>[4x]MTDYDLAKETAAWLNKQLQIRPVLGIVCGSGLGKIGDSLETSITVAYSDIPNFPVGSVKGHAGSLIFGSVNGVSCVCMKGRFHLYEGHTAARATFPMRVFKALGVKIV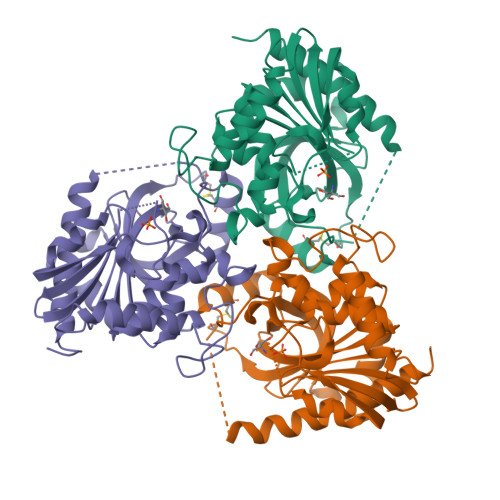VLTNAAGGLNPSYRPGDFMVVRDHINLPGLAGANPLTGPNDDTEGERFPSMTSVYDKTLRKYAISAARELGMSYATHEGVYCCVNGPSFETPAECKILRLMGSDAVGMSTAPETIVAKHGGMRCLAVSLISNVIASNCETPAEPTHEEVLRAGEEASARMTALVKLVIEKIRGELPR> GAGCAACUUAGGAUUUUAGGCUCCCCGGCGUGUCUCGAACCAUGCCGGGCCAAACCCAUAGGG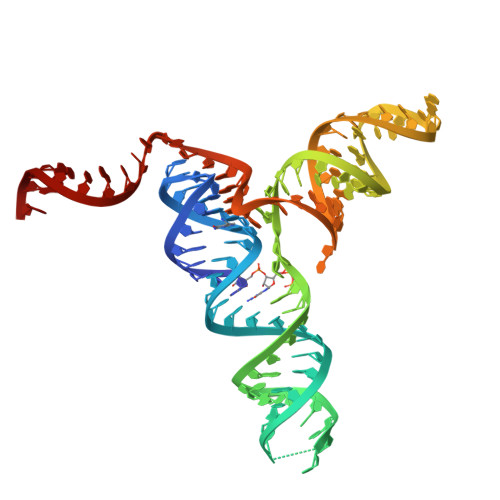CUGGCGGUCCCUGUGCGGUCAAAAUUCAUCCGCCGGAG> RTQSSTGTHGGYYYSFWTDNPNTVTYTNQNAGQFSVSWSGNQGNFVGGKGWNPGAARTIKYSGTYNPNGNSYLAVYG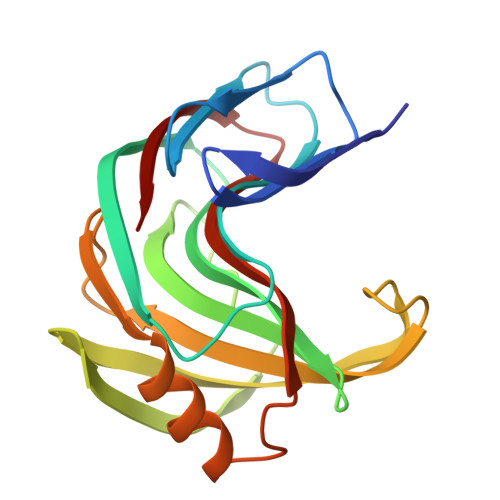WTRNPLIEYYIVENFGTYNPSSGATAAGEVTVDGSVYDIYTSTRTNAPSIEGTRTFQQYWSVRRNKRSSGSVNTGAHFNAWSNVGLALGSHDYQILAVEGYYSSGSATMTVS> RVEDLHVGATVAPSSRRDFTFDLYRALASAAPSQNIFFSPVSISMSLAMLSLGAGSSTKMQILEGLGLNLQKSSEKELHRGFQQLLQELNQPRDGFQLSLGNALFTDLVVDLQDTFVSAMKTLY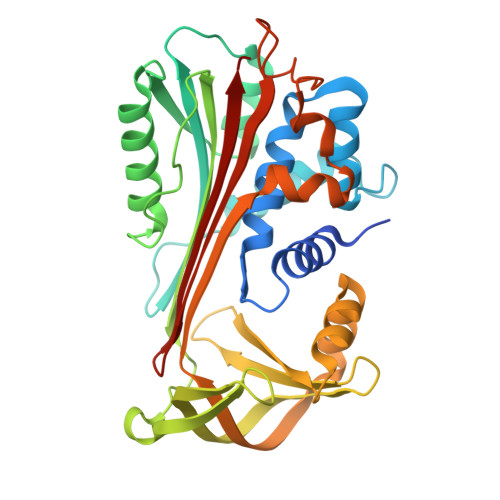LADTFPTNFRDSAGAMKQINDYVAKQTKGKIVDLLKNLDSNAVVIMVNYIFFKAKWETSFNHKGTQEQDFYVTSETVVRVPMMSREDQYHYLLDRNLSCRVVGVPYQGNATALFILPSEGKMQQVENGLSEKTLRKWLKMFKKRQLELYLPKFSIEGSYQLEKVLPSLGISNVFTSHADLSGISNHSNIQVSEMVHKAVVEVDESGTRAAAATGTIFTFRSA> MDQECIENYAKVNGIYIYYKLCKAPEEKAKLMTMHGGPGMSHDYLLSLRDMTKEGITVLFYDQFGCGRSEEPDQSKFTIDYGVEEAEALRSKLFGNEKVFLMGSSYGGALALAYAVKYQDHLKGLIVSGGLSSVPLTVKEMNRLIDELPAK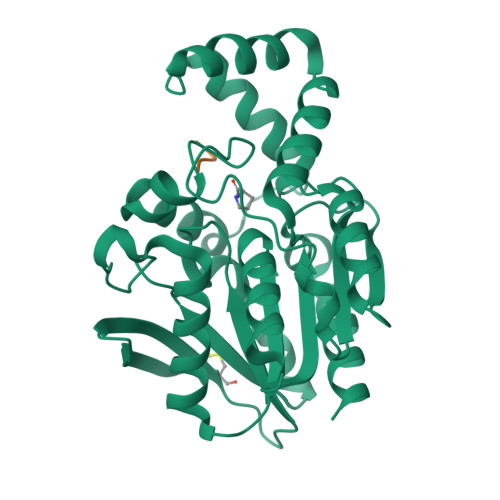YRDAIKKYGSSGSYENPEYQEAVNYFYHQHLLRSEDWPPEVLKSLEYAERRNVYRIMNGPNQFTITGTIKDWDITDKISAIKIPTLITVGEYDEVTPNVARVIHEKIAGSELHVFRDCSHLTMWEDREGYNKLLSDFILKHL;> PLGG> MQDNSRYTHFLTQHYDAKPQGRDDRYCESIMRRRGLTSPCKDINTFIHGNKRSIKAICENENGNPHRENLRISKSSFQVTTCKLHGGSPWPPCQYRATAGFRNVVVACENGL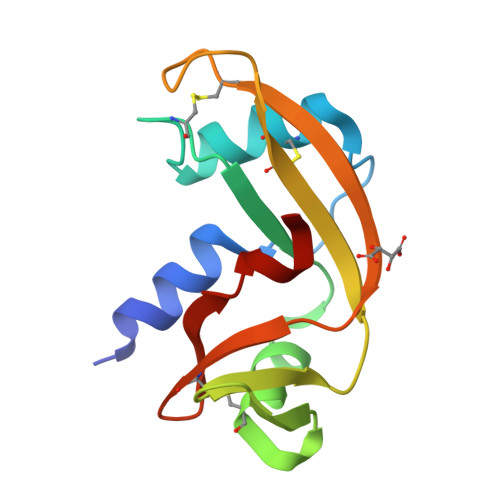PVHLDQSIFRRP>MTRIILPGKTIGIIGGGQLGRMMALAAKEMGYKIAVLDPTKNSPCAQVADIEIVASYDDLKAIQHLAEISDVVTYEFENIDYRCLQWLEKHAYLPQGSQLLSKTQNRFTEKNAIEKAGLPVATYRLVQNQEQLTEAIAELSYPSVLKTTTGGYDGKGQVVLRSEADVDEARKLANAAECILEKWVPFEKEVSVIVIRSVSGETKVFPVAENIHVNNILHESIVPARITEELSQKAIAYAKVLADELELVGTLAVEM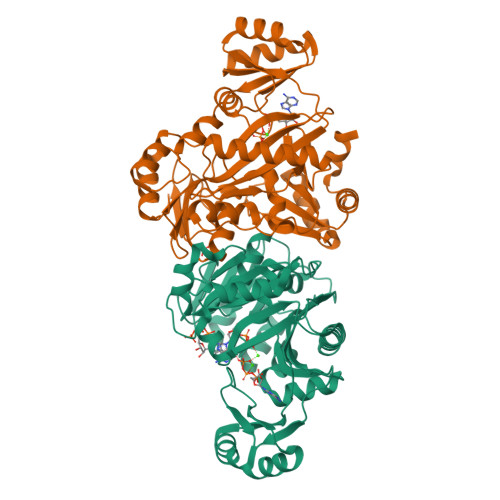FATADGEIYINELAPRPHNSGHYTQDACETSQFGQHIRAICNLPLGETNLLKPVVMVNILGEHIEGVLRQVNRLTGCYLHLYGKEEAKAQRKMGHVNILNDNIEVALEKAKSLHIWDHQEQLLE[2x]> DTHFPICIFCCGCCHRSKCGMCC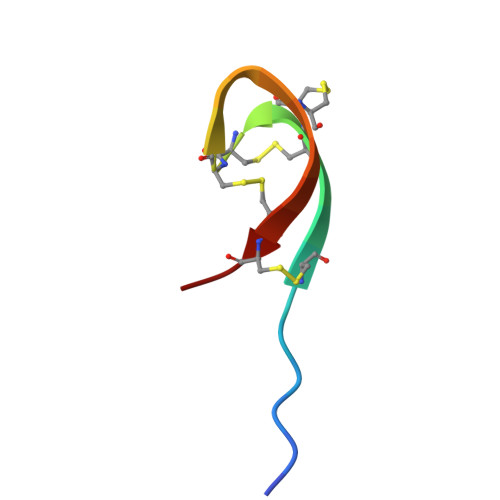KT> MLRVAGRRLFSVSQRSSTATSFVVSRDHTLSDGGGDSSSAPRSLPSADLSSYHRSLIRGFSSQVLAQGNEIGFGSEVPATVEAVKTPNSKIVYDDHNHERYPPGDPSKRAFAYFVLSG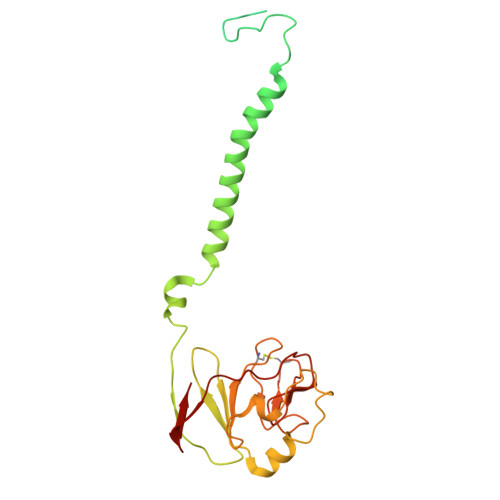GRFVYASVLRLLVLKLIVSMSASKDVLALASLEVDLGSIEPGTTVTVKWRGKPVFIRRRTEDDIKLANSVDVGSLRDPQEDSVRVKNPEWLVVVGVCTHLGCIPLPNAGDYGGWFCPCHGSHYDISGRIRKGPAPYNLEVPTYSFLEENKLLIG> ETGNQDLPVIKCVLINHKNNDSSVGKSSSYPMVSESPEDLGCALRPQSSGTVYEAAAVEVDVSASITLQVLVDAPGNISCLWVFKHSSLNCQPHFDLQNRGVVSMVILKMTETQAGEYLLFIQSEATNYTILFTVSIRNTLLYTLRRPYFRKMENQDALVCISESVPEPIVEWVLCDSQGESCKEESPAVVKKEEKVLHELFGTDIRCCARNELGRECTRLFTIDLNQTPQTTLPQLFLKVGEPLWIRCKAVHVNHGFGLTWELENKALEEGNYFEMSTYSTNRTMIRILFAFVSSVARNDTGYYTCSSSKHPSQSALVTIVEKGFINATNSSEDYEIDQYEEFCFSVRFKAYPQIRCTWTFSRKSFPCEQKGLDNGYSISKFCNHKHQPGEYIFHAENDDAQFTKMFTLNIRRKPQVLAEASASQASCFSDGYPLPSWTWKKCSDKSPNCTEEITEGVWNRKANRK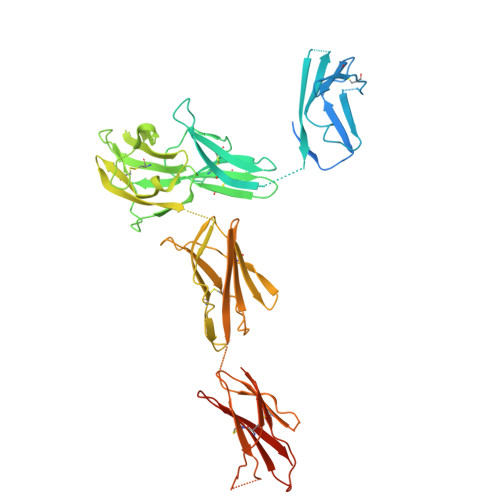VFGQWVSSSTLNMSEAIKGFLVKCCAYNSLGTSCETILLNSPGPFPFIQDGGTKHHHHHH>[5x]QDMVSPPPPIADEPLTVNTGIYLIECYSLDDKAETFKVNAFLSLSWKDRRLAFDPVRSGVRVKTYEPEAIWIPEIRFVNVENARDADVVDISVSPDGTVQYLERFSARVLSPLDFRRYPFDSQTLHIYLIVRSVDTRNIVLAVDLEKVGKNDDVFLTGWDIESFTAVVKPANFALEDRLESKLDYQLRISRQYFSYIPNIILPMLFILFISWTAFWSTSYE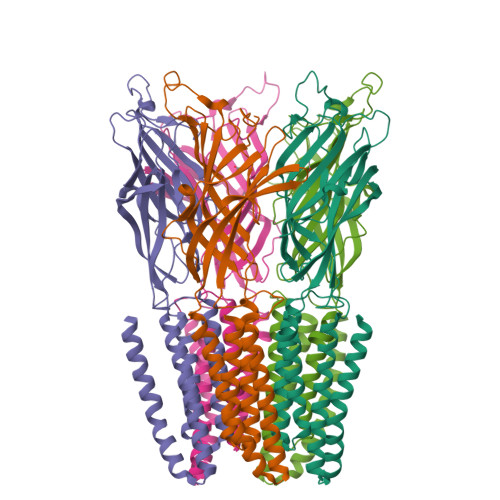ANVTLVVSTLIAHIAFNILVETNLPKTPYMTYTGAIIFMIYLFYFVAVIEVTVQHYLKVESQPARAASITRASRIAFPVVFLLANIILAFLFFGF>[4x]MHHHHHHSSGRENLYFQGIRMSQILEPRSEEDWTAHRTRIVCTMGPACWNVDTLVKMIDAGMNVCRLNFSHGDHETHARTVQNIQEAMKQRPEARLAILLDTKGPEIRTGFLKDHKPITLQQGATLKIVTDYNLIGDETTIACSYGALPQSVKPGNTILIADGSLSVKVVEVGSDYVITQAQNTATI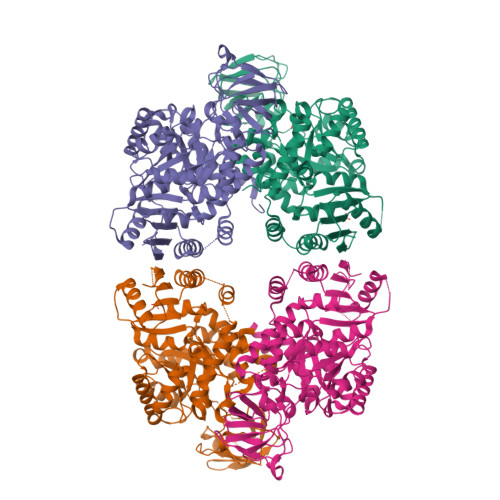GERKNMNLPNVKVQLPVIGEKDKHDILNFGIPMGCNFIAASFVQSADDVRYIRGLLGPRGRHIRIIPKIENVEGLVNFDEILAEADGIMIARGDLGMEIPPEKVFLAQKMMIAKCNVVGKPVITATQMLESMIKNPRPTRAEAADVANAVLDGTDCVMLSGETANGEFPVITVETMARICYEAETCVDYPALYRAMCLAVPPPISTQEAVARAAVETAECVNAAIILALTETGQTARLIAKYRPMQPILALSASESTIKHLQVIRGVTTMQVPSFQGTDHVIRNAIVVAKERELVTEGESIVAVHGMKEEVAGSSNLLKVLTVE> CGGAAATTC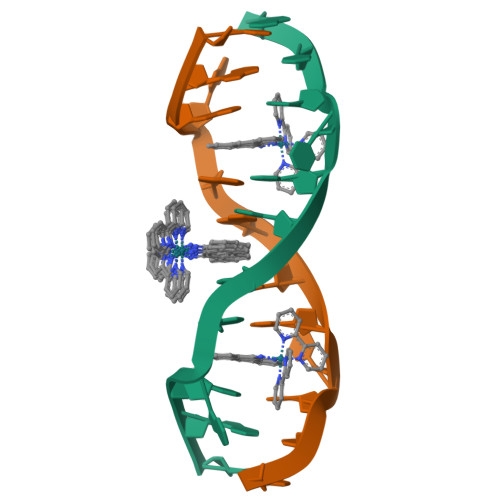CCG>MVKWRTLVHNGVALPPPYQPKGLSIKIRGETVKLDPLQEEMAYAWALKKDTPYVQDPVFQKNFLTDFLKTFNGRFQDVTINEIDFSEVYEYVERERQLKADKEYRKKISAERKRLREELKARYGWAEMDGKRFEIANWMVEPPGIFMGRGNHPLRGRWKPRVYEEDITLNLGEDAPVPPGNWGQIVHDHDSMWLARWDDKLTGKEKYVWLSDTADIKQKRDKSKYDKAEMLENHIDRVREKIFKGLRSKEPKMREIALACYLIDRLAMRVGDEKDPDEADTVGATTLRVEHVKLLEDRIEFDFLGKDSVRWQKSIDLRNEPPEVRQVFEELLEGKKEGDQIFQNINSRHVNRFLGKIVKGLTAKVFRTYIATKIVKDFLAAIPREKVTSQEKFIYYAKLANLKAAEALNHKRAPPKNWEQSIQKKEERVKKLMQQLREAESEKKKARIAERLEKAELNLDLAVKVRDYNLATSLRNYIDPRVYKAWGRYTGYEWRKIYTASLLRKFKWVEKASVKHVLQYFAEKLAKDVDKGMQVKAAV[2x]

Type IB topoisomerases (Topo IB) are found in all eukaryotes (where they are referred to as TOP1), in several archaeal phyla, several bacterial genera and several groups of viruses. TOP1, also known as swivelase or untwisting enzyme, can relax both positive and negative supercoils by nicking DNA, enabling the rotation of the broken DNA strand around the complementary intact strand of the DNA duplex and catalyzing the closing of the nick. In particular, one topoisomerase from the hyperthermophilic archaeon Caldiarchaeum subterraneum (CsTOP1) was found to be highly similar to human TOP1 (34% sequence identity, 53% similarity) and to display similar activity, while being extremely stable. Here, we solved the structure of thermostable archaeal Caldiarchaeum subterraneum CsTOP1 in an apo-form.

We solved the crystal structure of both selenomethionine-labelled (SeMet) CsTOP1 and native CsTOP1 at 2.0 and 2.20 Å, respectively. In both cases, the asymmetric unit of the crystal contained two TOP1 molecules. In the asymmetric unit, each TOP1 molecule folds similarly, and there is no significant difference between SeMet CsTOP1 and native CsTOP1. In its apo-form, CsTOP1 folds as a compact protein, comprised of the CAP region (1–207), the CAT region (208–412), the linker (413–469), and the C-terminal region (469–524). The electron density of the C-terminal extremity of CsTOP1 (525–539) is not visible in these crystal structures, suggesting that this region, which is poorly conserved in other archaea, is flexible. The enzyme displays an open conformation resulting from one substantial rotation between the capping (CAP) and the catalytic (CAT) modules. In the apo-form structure, the TOP1 CAP domain does not block access of the DNA molecule to the DNA interacting region. The Lip2 loop segment moves towards this region and partially covers it. More precisely, the side chain of glutamate Glu278 (Lip2) forms hydrogen bonds with the Nε atom of His410 and the hydroxyl group of Tyr477. Therefore, while the DNA cavity is not blocked by the presence of the CAP domain in the CsTOP1 open-conformation, the Lip2 loop interaction with the catalytic tetrad may hinder the entry of the DNA molecule, and its displacement seems necessary for DNA binding.>SNAMKVTDVRLRKIQTDGRMKALVSITLDEAFVIHDLRVIEGNSGLFVAMPSKRTPDG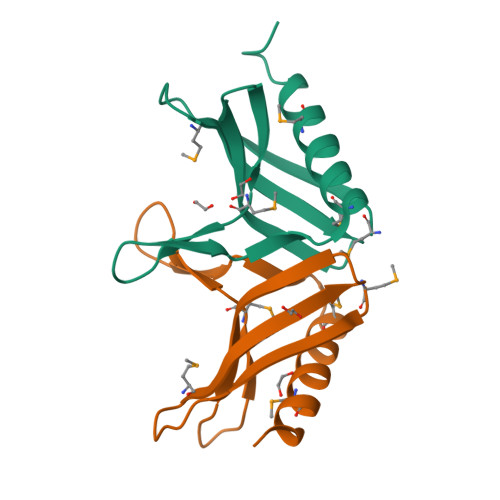EFRDIAHPINSDMRQEIQDAVMKVYDETDEVIPDKNATSDNEESDEA[2x]>[2x]SATTPPGDLEQPELEARVKEIIEVDGYQFRDLNDNGELDPYEDWRLPTPERVADLVGQMSLVEKSGLMLINTLNAACDPQTGEFGVLPAQADNYINTQHMHRFVFRNVVDVRAEGVECTGTGTPVVSPAEAATFTNAVQEMSEATRLGIPSLFKSNARNHIDPDARVGINEAAGAFSAFPKEAGIAAAALGEQARRTGEATTGDMSVVADFADVMGEEWASIGLRGMYGYMADLSTEPRWYRTHETFTEDAYLAAEIMETLVQTL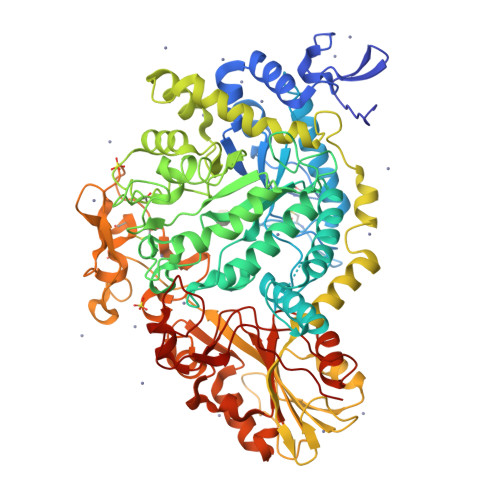QGEELTDNGLALSPQTRVALTLKHFPGGGPQELGLDPHYAFGKAQVYPAGRFEEHFLPFQAAIDAGVSSIMPYYGVPVDVPVVGGEPGETYPHTGFAFSDSIVNGLLRDQLGFTGYVNSATGIINDRAWGLEGNTVPERVAAAINGGTDTLSGFSDVSVITDLYEADLISEERIDLAAERLLEPLFDMGLFENPYVDPDVATATVGADDHRAVGLDLQRKSLVLLQNEETDEGPVLPLKEGGDVYILGDFTEETVESYGYEVTNGNVAEGEERPSAAGSDYVLISMTAKTNAGDYVSDDPSLGLNPDHGTNPSVIIGDDGEPLPGLDGQSLWGAADVCVHKEGHEENPSCTDNRLRFGGAYPWESSILDFTGMEAAESWEVVPSLETIQEVMAEVEDPSKVILHVYFRQPYVLDEESGLRDAGAILAGFGMTDTALMDVLTGAYAPQGKLPFALAGTREAIIEQDSDRPGYDETEDGALYPFGYGLTYEDDTEE> MAHHHHHHVDDDDKMVHHDGFQTVKATIDWEHPMFKLYEKAKRNGKWNPADIDFSQDQKDFASLTSEEKISALPLVAGFSAGDEAVTLDILPMAHALARQGRLEDVLFLTTFMHDEAKHVEMFSRWQQAVGIGQMDLSVFHNDHYKRIFYEALPEAMNRLYADDSPEAVIRAATVYNMIVEGTLAESGYYTFRQIYKKAGLFPGLLQGIDYLNMDEGRHIQFGIYTIQRIVNEDERYYELFIRYMDELWPHVIGYVDYLTELGK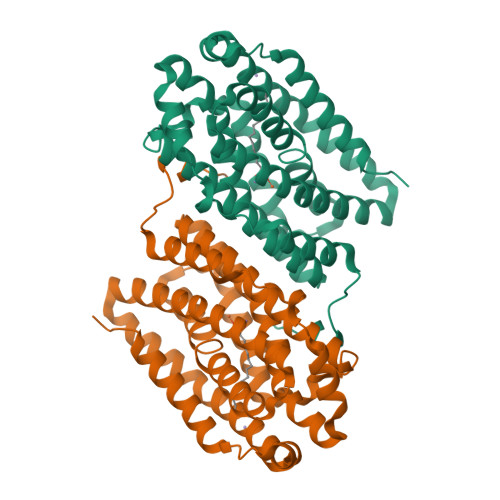RQQQLARTYALEIDYDLLRHYVIKQFNLRKKQISRTKRVDVVEGLEKTAAES>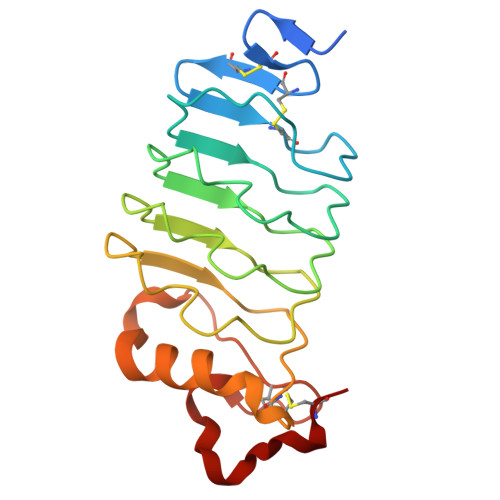 GGHHHHHHGSENLYFQGACPSQCSCSGTTVDCSGKSLASVPGGIPTTTQVLYLYDNQITKLEPGVFDRLVNLQQLWLEINQLTSLPAGVFDNLTQLSILNMHTNQLKSIPRGAFDNLKSLTHIWLLNNPWDCACSDILYLSGWLGQHAGKEQGQAVCSGTNTPVRAVTEASTSPSKCP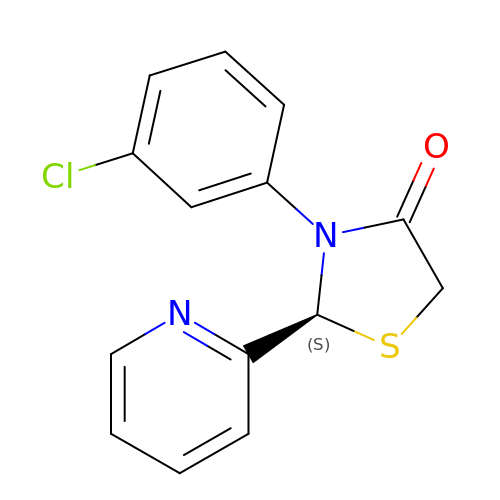(2S)-3-(3-chlorophenyl)-2-(pyridin-2-yl)-1,3-thiazolidin-4-one | C14 H11 Cl N2 O S | XBARGMZJUZLYLI-AWEZNQCLSA-N> MAPSRANTSVIVVGGGGTIGSSTALHLVRSGYTPSNVTVLDAYPIPSSQSAGNDLNKIMGVSLRNPVDLQLALEARQMWNEDELFKKFFHNTGRLDCAHGEKDIADLKSGYQALVDAGLDATNEWLDSEDEILKRMPLLSRDQIKGWKAIFSKDGGWLAAAKAINAVGEYLRDQGVRFGFYGAGSFKAPLLAEGVCIGVETVDGTRYYADKVVLAAGAWSPTLVELHEQCVSKAWVYGHIQLTPEEAARYKNSPVVYNGDVGFFFEPNEHGVIKVCDEFPGFTRFKMHQPFGAKAPKRISVPRSHAKHPTDT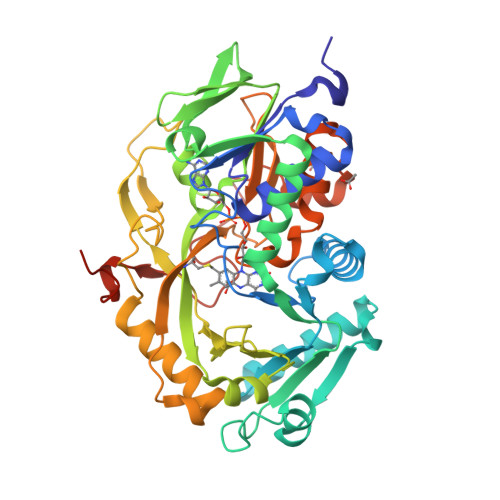IPDASDVSIRRAIATFMPQFKNKKMFNQAMCWCTDTADAALLICEHPEWKNFVLATGDSGHSFKLLPNIGKHVVELLEGTLADDLAHAWRWRPGSGDALKSRRSAPAKDLADMPGWNHDKPRANLLEHHHHHH> MKKQKRTQGKQNTKQIKQEKLSSKRKANNQKEGKKKVKQEDYKEIKQKGKRMLSKIVKASFSSKGFNLANAVNTVKSTLNAPIKHIKRNIEPTGSNYSRMTNTTEEAFDEVSHEWQALVTSNPFDLNVFNYLENTQTSNFGTVDNPLVVFTSETPFRYVGCTGQMNEDDYEGHELLFFLLREGSLQRCMGCGQVFKLVRLRNEYSPEMDYYLSNFHPYEMQEMGESDTTVLMSPYKYASHYEYTQFETPSNMVYSMVNPDEHDRLLVDPAYRMERTKALEEKYKVYTSSLREVEKQFEERYGRAGQINISKVTYSTL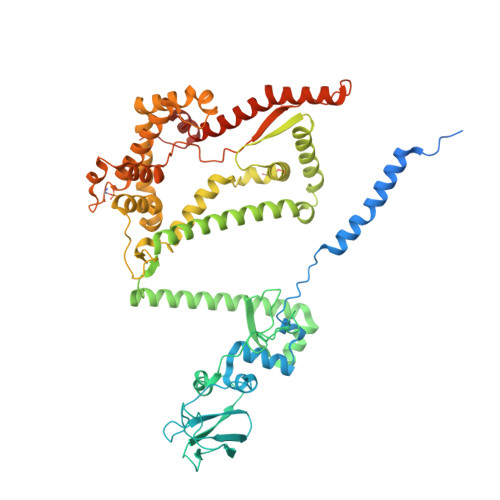IDVEKAVLKMDRLFRKVAKFENRAFIDRANHSRREKRMLERAQQRWDSNYSFFTGSLTEEEQKYRDYYETELEAYPEDEGIEQQLDQQEVLLSGRYDPKLYDFQEGYTKNPEDDQTSLIEKKAFKFRYRLANETSETFQRRNNRMVERQIKRFQQPQYKHAFEQLQKNIAISSNSGNALHSEYGYLELLSNESVQLYKDYYESDAEEDFKVFENLSSKEKLVMIANFENNLLPKYDRSEVHLIPKRQWEPAFGVWENFLYDITEYASFIAPRGKEIAADYQIQSAIPLTKEELIEAGLYKETIEKKVEPKLEAKKQTKSE> MRLELPVIPLRNTVILPHTTTPVDVGRAKSKRAVEEAMGADRLIFLVAQRDPEVDDPAPDDLYTWGVQAVVKQAMRLPDGTLQVMVEARARAQVTDYIPGPYLRARGEVFSEIFPIDEAVVRVLVEELKEAFEKYVAN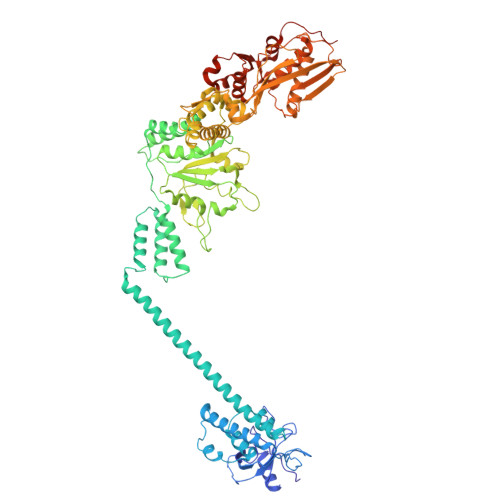HKSLRLDRYQLEAVKGTSDPAMLADTIAYHATWTVAEKQEILELTDLEARLKKVLGLLSRDLERFELDKRVAQRVKEQMDTNQREYYLREQMKAIQKELGGEDGLSDLEALRKKIEEVGMPEAVKTKALKELDRLERMQQGSPEATVARTYLDWLTEVPWSKADPEVLDINHTRQVLDEDHYGLKDVKERILEYLAVRQLTQGLDVRNKAPILVLVGPPGVGKTSLGRSIARSMNRKFHRISLGGVRDEAEIRGHRRTYIGAMPGKLIHAMKQVGVINPVILLDEIDKMSSDWRGDPASAMLEVLDPEQNNTFTDHYLDVPYDLSKVFFITTANTLQTIPRPLLDRMEVIEIPGYTNMEKQAIARQYLWPKQVRESGMEGRIEVTDAAILRVISEYTREAGVRGLERELGKIARKGAKFWLEGAWEGLRTIDASDIPTYLGIPRYRPDKAETEPQVGTAQGLAWTPVGGTLLTIEVAAVPGSGKLSLTGQLGEVMKESAQAALTYLRAHTQDYGLPEDFYNKVDLHVHVPDGATPKDGPSAGITMATAIASALSRRPARMDIAMTGEVSLRGKVMPIGGVKEKLLAAHQAGIHKIVLPKDNEAQLEELPKEVLEGLEIKLVEDVGEVLEYLLLPEPTMPPVVQPSDNRQQPGAGA> HGSPVDICTAKPRDIPMNPMCIYRSPEKKATEDEGSEQKIPEATNRRVWELSKANSRFATTFYQHLADSKN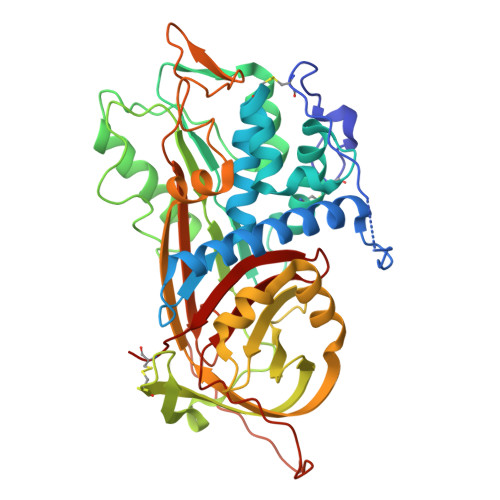DNDNIFLSPLSISTAFAMTKLGACNDTLQQLMEVFKFDTISEKTSDQIHFFFAKLNCRLYRKAQKSSKLVSANRLFGDKSLTFNETYQDISELVYGAKLQPLDFKENAEQSRAAINKWVSNKTEGRITDVIPSEAINELTVLVLVNTIYFKGLWKSKFSPENTRKELFYKADGESCSASMMYQEGKFRYRRVAEGTQVLELPFKGDDITMVLILPKPEKSLAKVEKELTPEVLQEWLDELEEMMLVVHMPRFRIEDGFSLKEQLQDMGLVDLFSPEKSKLPGIVAEGRDDLYVSDAFHKAFLEVNEEGCEAAASTAVVIAGRSLNPNRVTFKANRPFLVFIREVPLNTIIFMGRVANPCVK>MVMAILYTGPTGNGRKPLVLGKLLNAPIKVHMFHWPTKDIQEDWYLKLNPAGIVPTLVDDKGTPITESNNILLYIADTYDKEHKFFYSLKQDPKLYWEQNELLFYQATQFQSQTLTIANANYQNGHIDENIAQYVLSSFEKVFAFMETKLSGRDWFVGDKFTIVDIAFLVGEHRRRERLHNSPIWIDLKENFPNVEKWFQRAIAFENVEEILKEHAAEN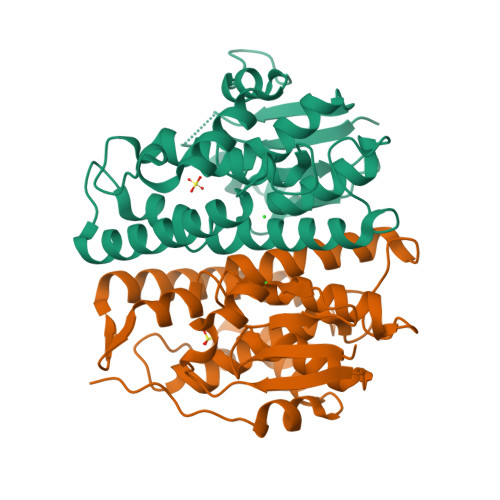LYFQSHHHHHHWSHPQFEK[2x]> G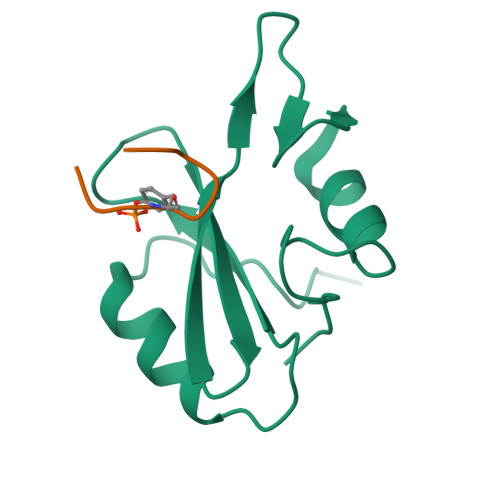SMAWFFGKIPRAKAEEMLSKQRHDGAFLIRESESAPGDFSLSVKFGNDVQHFKVLRDGAGKYFLWVVKFNSLNELVDYHRSTSVSRNQQIFLRDI;> APSYVNVQN>[4x]AVKVGINGFGRIGRNVFRAALKNPDIEVVAVNDLTDANTLAHLLKYDSVHGRLDAEVSVNGNNLVVNGKEIIVKAERDPENLAWGEIGVDIVVESTGRFTKREDAAKHLEAGAKKVIISAPAKNEDITIVMGVNQDKYDPKAHHVISNASCTTNCLAPFAKVLHEQFGIVRGMMTTVHSYTNDQRILDLPHKDLRRARAAAESIIPTTTGAAKAVALVLPELKGKLNGMAMRVPTPNVSVVDL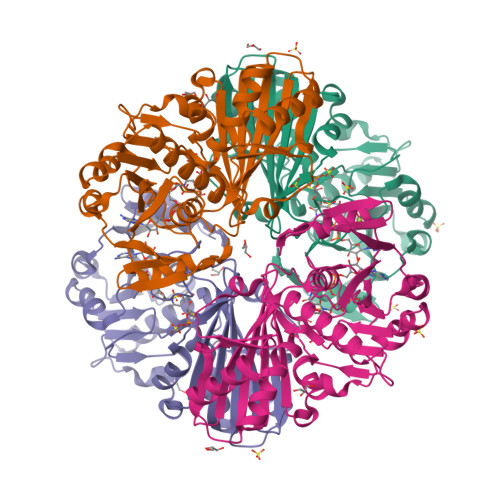VAELEKEVTVEEVNAALKAAAEGELKGILAYSEEPLVSRDYNGSTVSSTIDALSTMVIDGKMVKVVSWYDNETGYSHRVVDLAAYIASKGL>[4x]ALTYRGVDWSSVVVEERAGVSYKNTNGNAQPLENILAANGVNTVRQRVWVNPADGNYNLDYNIAIAKRAKAAGLGV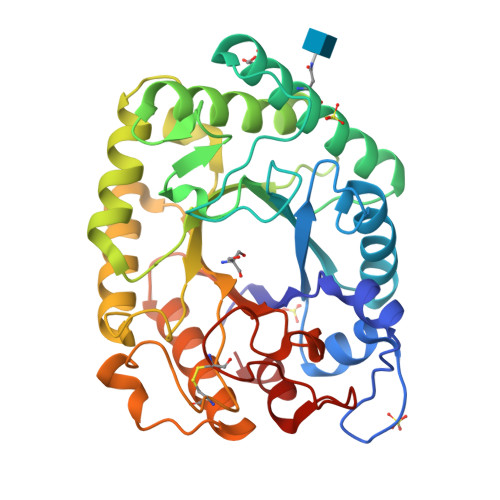YIDFHYSDTWADPAHQTMPAGWPSDIDNLSWKLYNYTLDAANKLQNAGIQPTIVSIGNEIRAGLLWPTGRTENWANIARLLHSAAWGIKDSSLSPKPKIMIHLDNGWDWGTQNWWYTNVLKQGTLELSDFDMMGVSFYPFYSSSATLSALKSSLDNMAKTWNKEIAVVETNWPISCPNPRYSFPSDVKNIPFSPEGQTTFITNVANIVSSVSRGVGLFYWEPAWIHNANLGSSCADNTMFSQSGQALSSLSVFQRI>[2x]GLEEEARELAEEAREVR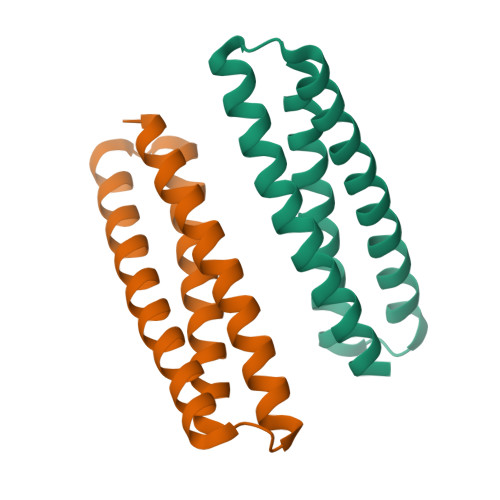RRAEELRRRAEEARETGEASEEHAAALLAEAAVLELKAVLLELEARRLLKESGGEVAREALELAREARREAREALEAAEEASE>GPGLKQKIVIKVAMEGNNCRSKAMALVASTGGVDSVALVGDLRDKIEVVGYGIDPIKLISALRKKVGDAELLQVS[2x]

NLRs are a conserved component of plants' innate immune systems and survey the host environment for perturbations caused by invading pathogens. Intriguingly, the NLR pair Pik-1/Pik-2, which recognises AVR-Pik, also binds the effector via an HMA domain but this domain is integrated between the CC and NB-ARC regions of Pik-1. The integrated HMA domains of RGA5 and Pik-1 appear to have evolved from a family of rice proteins that only contain the HMA domain. Each of the Pikp-HMA monomers adopts the HMA-domain fold (Pfam: PF00403), comprising a four-stranded antiparallel β-sheet and two α-helices packed in an α/β sandwich.

The closest structural homologue of Pikp-HMA (defined by PDBeFold [Krissinel and Henrick, 2004]) is the HMA domain of yeast protein Ccc2A, overlaying with an r.m.s.d. of 1.58 Å over 72 residues. Typically, HMA domains bind heavy metals, or lighter cations such as Cu1+ or Zn2+, via two conserved Cys residues and are involved in metal transport or detoxification pathways. Interestingly, these Cys residues are not conserved in Pik-1 HMA domains, including Pikp-1. Hence, the Pikp-HMA structure does not contain a metal ion, and the loop between β1 and α1, which usually contains the metal-chelating Cys residues, is disordered. The absence of obvious enzymatic activity in the effectors, and a lack of large conformation changes in Pikp-HMA in the AVR-PikD-bound and unbound states, supports the hypothesis that effector binding promotes domain re-arrangements in NLR complexes.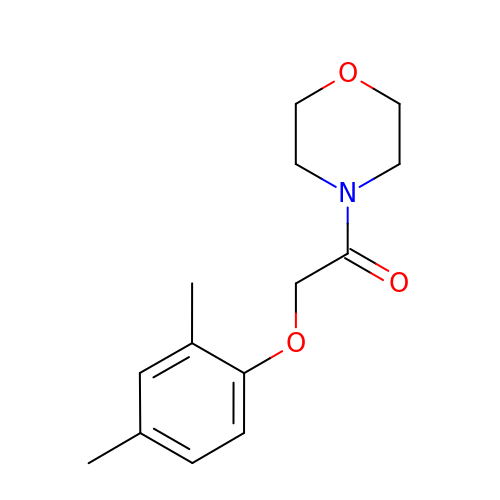2-(2,4-dimethylphenoxy)-1-morpholin-4-yl-ethanone | C14 H19 N O3 | SPKPARPPRVMDOW-UHFFFAOYSA-N6-{[(2,5-DIETHOXYPHENYL)AMINO]METHYL}-5-METHYLPYRIDO[2,3-D]PYRIMIDINE-2,4-DIAMINE | C19 H24 N6 O2 | 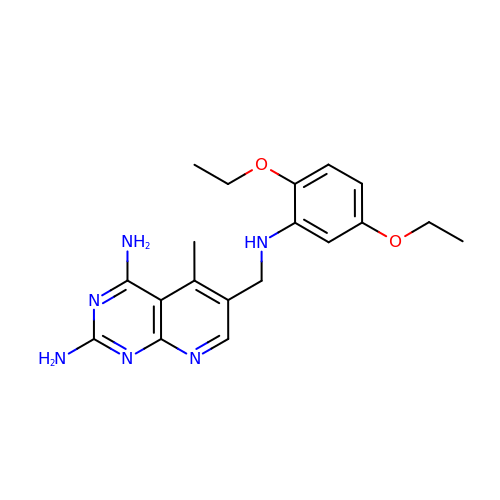KKMWDWUZXFYKLD-UHFFFAOYSA-N>MHHHHHHGVLKSPPPMPKLDLEEWWGPPELKQKQDTSIKPFEITFSETMVKELKERIKKRRPFAPPLEGVGFKYGFNSKQLDSWLKYWAEEYPFAERQKFLNQYPHFKTNIQGLNIHFMRITPKVPKGVEIVPLLLLHGWPGSVREFYEAIPHLTAVSKDRNFALEIIAPSLPGYGFSDAAVRPGLAAAEVAVIFKNLMARLGYKQYYVQGGDWGALIGSAMATFFPKEIIGFHSNMALTLSPAATFLEFVGALFPSLIVEPELANRLYPLSEKYSTLLEELGYMHIQATKPDTVGIGLTDSPAGLLAYILEKFSTWTNPDLRSKEDGGLSYRWT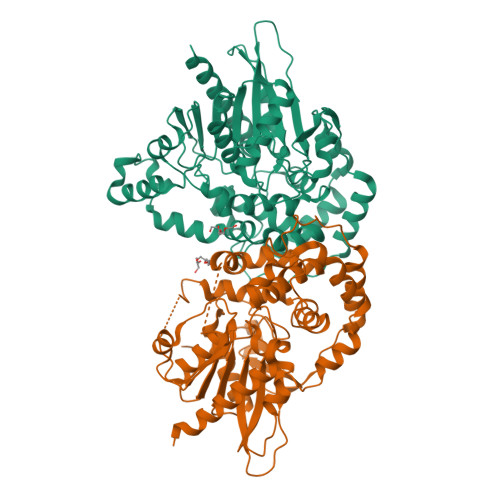KDQLIDNLMLYWSTKSIVTSMRLYAESFSSRHFDLKLDEIQVQVPTWVLQAKHELAYQPPCILKMKYPKLVNASVIEDGGHFLAFELPEIFAKDVLKAIGEFRKLKNVKTEL[2x]> FDVNSHTTPCGPVTCSGAQMCEVDKCVC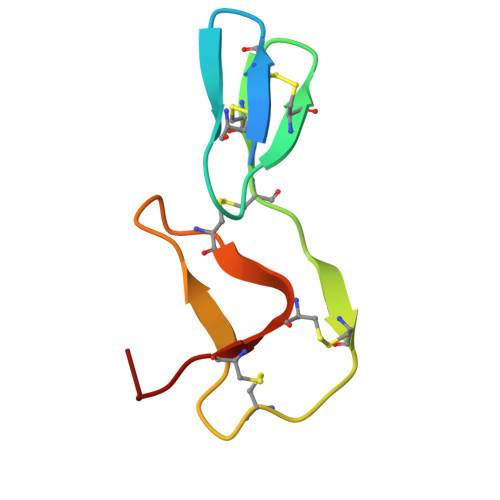SDLHCKVKCEHGFKKDDNGCEYACICADAPQ We used de novo protein design to generate very closely related proteins that adopt two very different states—a short state and a long state, like a viral fusion protein—and then created a single molecule that can be found in both forms. Inspired by class I viral fusion proteins, such as influenza hemagglutinin, we chose homotrimeric helical bundles as the fundamental architecture. We decided on a design scheme with two divergent conformations containing a constant six-helix bundle “base” and a variable portion with three inner helices and three “flipping” helices. In the compact “short” state (∼66 Å height), the flipping helices fold back to interact with the inner helices; in the extended “long” state (∼100 Å height), they extend to form interactions with each other.

The interaction energy between the flipping helix and the inner helices in the short state was tuned by combining hydrogen bond layers (“A”) or hydrophobic layers (“X”) in different orders in each of three possible positions. Designs were given three-letter names corresponding to the layers in order, starting at the hinge proximal position. Structure prediction calculations (Rosetta symmetric fold-and-dock) suggested that some layer combinations (such as XAX) would be more favorable for the short state than others (such as AAA) and that the short and long backbones states would be among the lowest-energy states of these systems. SEC-MALS measurements indicated that, in solution, XAX, XAA, and AAA were trimeric as expected; CD wavelength and temperature measurements for XAX, XAA, and AAA showed that the designs were helical and highly temperature stable. The number and position of the hydrogen bond networks appears to determine the state which is populated—designs with one network folding into the short state, with two networks, into a more dynamic short state, and with three networks, into the long state. The hydrogen-bond network residues were closer to the computational model in XAX than in XXA, likely because they were buried in the former and solvent exposed in the latter. By NMR, the average solution structure adopted by XAX was locked in the compact state, as shown by the presence of multiple NOEs from a 3D CM-CMHM nuclear Overhauser enhancement spectroscopy (NOESY) spectrum.

>GSHMGTEDLKYSLERLREILERLEENPSEKQIVEAIRAIVENNAQIVEAIRAIVEILALIVENNRAIIEALEAIGGGTKILEEMKKQLKDLKRALERG[3x]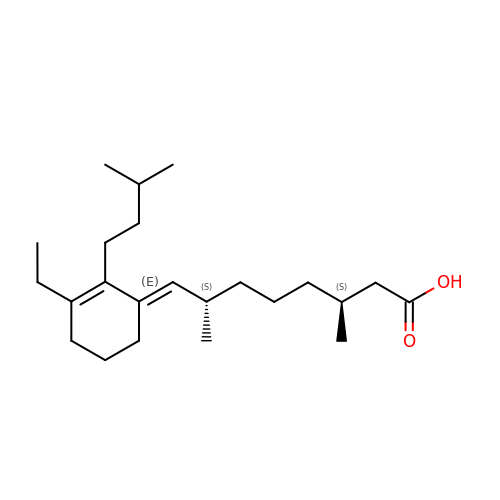(3S,7S,8E)-8-[3-ethyl-2-(3-methylbutyl)cyclohex-2-en-1-ylidene]-3,7-dimethyloctanoic acid | C23 H40 O2 | XIXDFZCDSAMZDB-AQOSXKMFSA-N>GAMGDFSFIKALQTAQQNFVVTDPSLPDNPIVYASQGFLNLTGYSLDQILGRNCRFLQGPETDPKAVERIRKAIEQGNDMSVCLLNYRVDGTTFWNQ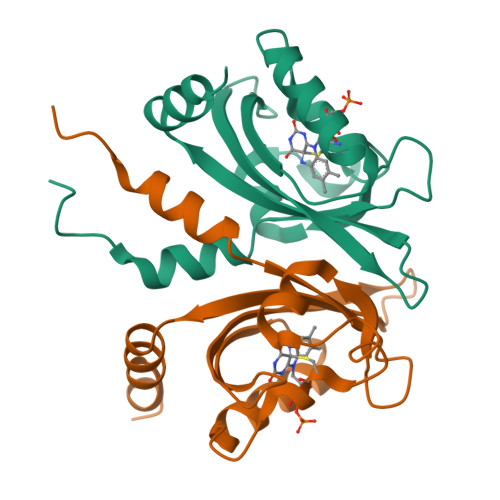FFIAALRDAGGNVTNFVGVQCKVSDQYAATVTKQQEEEEEAAANDDED[2x]>MDYEILFSDETMNYADAGTYCQSRGMALVSSAMRDSTMVKAILAFTEVKGHDYWVGADNLQDGAYNFLWNDGVSLPTDSDLWSPNEPSNPQSWQLCVQIWSKYNLL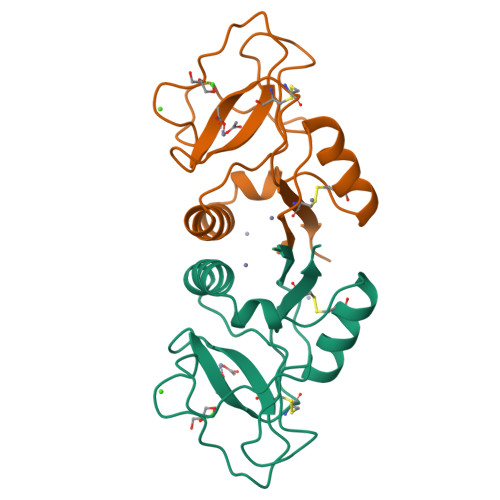DDVGCGGARRVICEKELDD[2x]The mitochondrial disulfide relay is mediated within the mitochondrial intermembrane space (IMS) by the CHCHD4/MIA40 chaperone, itself a member of the CHCH family. Among more complex eukaryotes, however, the CHCHD4 N-terminus lacks this mitochondria-targeting membrane tether and instead forms an NAD(H)-regulated complex with IMM-anchored oxidoreductase Apoptosis-Inducing Factor (AIF). NADH is known to allosterically stimulate AIF dimerization and release a 50-residue disordered loop from AIF’s surface by reducing and forming a stable charge-transfer complex (CTC) with AIF’s FAD cofactor. Here we find that CHCHD4’s scaffolding of dimeric AIF unveils a dedicated, NAD(H)-regulated import platform within the IMS that anchors and orients CHCHD4 to encounter incoming substrates, while also unshielding the CHCHD4 active site to stimulate disulfide chaperone activity.

To generate a stable complex for crystallization, we engineered a custom construct linking CHCHD4’s N-terminal interaction domain (N45) to the dimer-permissive AIF (104-613) W196A mutant which maintains an open C-loop. The AIF-CHCHD4 chimera crystallizes in conditions resembling the original AIF-W196A mutant, allowing the structure to be solved by molecular replacement. The structure reveals the expected conserved AIF dimer. The CHCHD4 N-terminal domain is resolved for both AIF monomers, allowing the first 30 (Molecule 1) and 20 (Molecule 2) residues, respectively, to be modeled into the electron density. The structure reveals that the dissociation of AIF’s C-loop exposes a unique binding surface, allowing CHCHD4 to form a hydrophobic scaffold around AIF’s C-terminal domain. The CHCHD4 N-terminus assumes a unique β-hairpin/helix motif when complexed with AIF with a buried solvent accessible surface area of 1440 Å. The first twenty residues form a β-hairpin, which pairs with the core β-sheet of AIF’s C-terminal domain in a parallel orientation. The interface with AIF is mediated by hydrophobic side chains of β-hairpin residues I12, I13, F14, and V15 which complement the exposed hydrophobic edge of AIF’s C-terminal domain. The helical turn is anchored by a histidine (H20) which inserts into a hydrophobic pocket formed by AIF residues I610, V507, V564, and A604 and makes a water-mediated contact with N602. C-loop boundary residues F508 and Y560 contribute to AIF’s hydrophobic binding surface, forming an aromatic tetrad with Y347 and W351 as previously observed in crystal structures of the activated AIF dimer.

>[2x]MLTPEQKQKKAALSASEGEEVPQDKAPSHVPFLLIGGGTAAFAAARSIRARDPGARVLIVSEDPELPYMRPPLSKELWFSDDPNVTKTLRFKQANGKERSIYFQPPSFYVSAQDLPHIENGGVAVLTGKKVVQLDVRDNMVKLNDGSQITYEKCLIATGGTPRSLSAIDRAGAEVKSRTTLFRKIGDFRSLEKISREVKSITIIGGGFLGSELACALGRKARALGTEVIQLFPEKGNMGKILPEYLSNWTMEKVRREGVKVMPNAIVQSVGVSSGKLLIKLKDGRKVETDHIVAAVGLEPNVELAKTGGLEIDSDFGGFRVNAELQARSNIWVAGDAACFYDIKLGRRRVEHHDHAVVSGRLAGENMTGAAKPYWHQSMFWSDLGPDVGYEAIGLVDSSLPTVGVFAKATAQDNPKSATEQSGTGIRSESETESEASEITIPPSTPAVPQAPVQGEDYGKGVIFYLRDKVVVGIVLWNIFNRMPIARKIIKDGEQHEDLNEVAKLFNIHEDSGSGPGSGSMSYCRQEGKDRIIFVTKEDHETPSSAELVADDPNDPYEEHGLILPLEVLFQ>[2x]SNSITENTSWNKEFSAEAVNGVFVLCKSSSKSCATNDLARASKEYL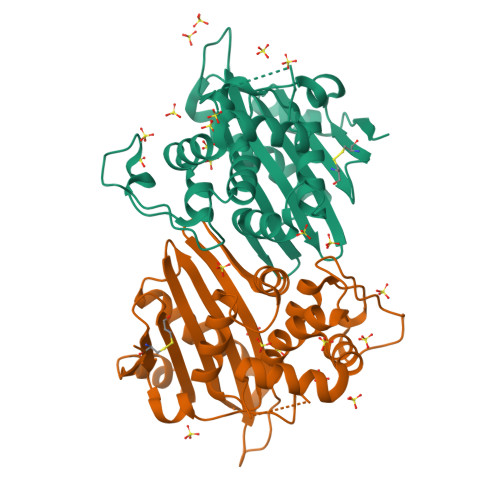PASTFKIPNAIIGLETGVIKNEHQVFKWDGKPRAMKQWERDLTLRGAIQVSAVPVFQQIAREVGEVRMQKYLKKFSYGNQNISGGIDKSWLEDQLRISAVNQVEFLESLYLNKLSASKENQLIVKEALVTEAAPEYLVHSKTGFSGVGTESNPGVAWWVGWVEKETEVYFFAFNMDIDNESKLPLRKSIPTKIMESEGIIGG> UC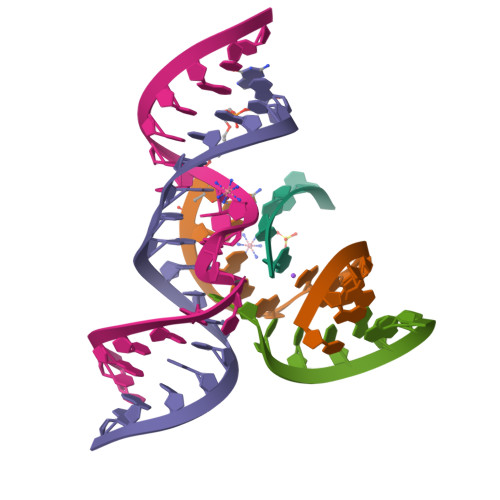CCA;> CGGUGAGAAGGGX;> GGCAGAGAAACACACGA;> UCGUGGUACAUUACCUGCC;> GUCCACCG>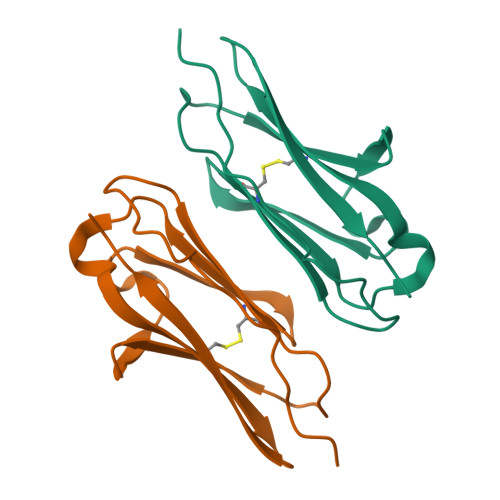[4x]GASGSVPPSIAPFSFGDDPVNTGENAGVQCMVQKGDVPITIKWTLNSRPIINGEEGITILKLSPKTSVLNIAAVEQDHRGVFKCIAENKAGSSFTTSELKVN>[2x]MARKLFTPITIKDMTLKNRIVMSPMCMYSSHEKDGKLTPFHMAHYISRAIGQVGLIIVEASAVNPQGRITDQDLGIWSDEHIEGFAKLTEQVKEQGSKIGIQLAHAGRKAELEGDIFAPSAIAFDEQSATPVEMSAEKVKETVQEFKQAAARAKEAGFDVIEIHAAHGYLIHEFLSPLSNHRTDEYGGSPENRYRFLREIIDEVKQVWDGPLFVRVSASDYTDKGLDIA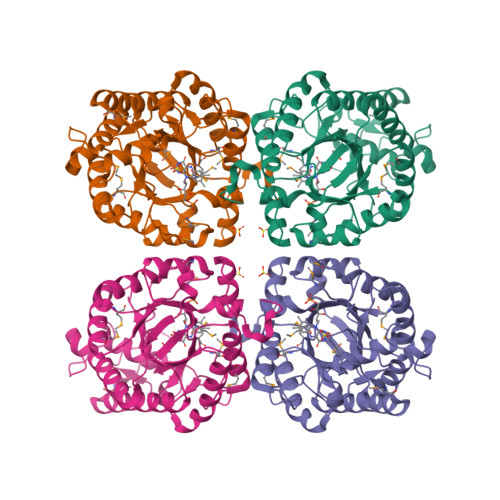DHIGFAKWMKEQGVDLIDCSSGALVHADINVFPGYQVSFAEKIREQADMATGAVGMITDGSMAEEILQNGRADLIFIGRELLRDPFFARTAAKQLNTEIPAPVQYERGW> GTRSESTEGHSKDLLYKYKLYGDIDEYAYYFLDIDIGTPEQRISLILDTGSSSLSFPCAGCKNCGVHMENPFNLNNSKTSSILYCENEECPFKLNCVKGKCEYMQSYCEGSQISGFYFSDVVSVVSYNNERVTFRK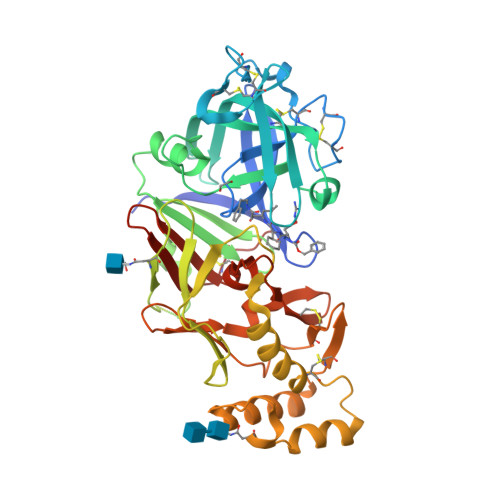LMGCHMHEESLFLYQQATGVLGMSLSKPQGIPTFVNLLFDNAPQLKQVFTICISENGGELIAGGYDPAYIVRRGGSKSVSGQGSGPVSESLSESGEDPQVALREAEKVVWENVTRKYYYYIKVRGLDMFGTNMMSSSKGLEMLVDSGSTFTHIPEDLYNKLNYFFDILCIQDMNNAYDVNKRLKMTNESFNNPLVQFDDFRKSLKSIIAKENMCVKIVDGVQCWKYLEGLPDLFVTLSNNYKMKWQPHSYLYKKESFWCKGIEKQVNNKPILGLTFFKNRQVIFDIQKNRIGFVDANCPSHPTHTRPR> DPRNLPIRQQMEALIRRKQAEITQGLESIDTVKFHADTWTRGNDGGGGTSMVIQDGTTFEKGGVNVSVVYGQLSPAAVSAMKADHKNLRLPEDPKTGLPVTDGVKFFACGLSMVIHPVNPHAPTTHLNYRYFETWNQDGTPQTWWFGGGADLTPSYLYEEDGQLFHQLHKDALDKHDTALYPRFKKWCDEYFYITHRKETRGIGGIFFDDYDERD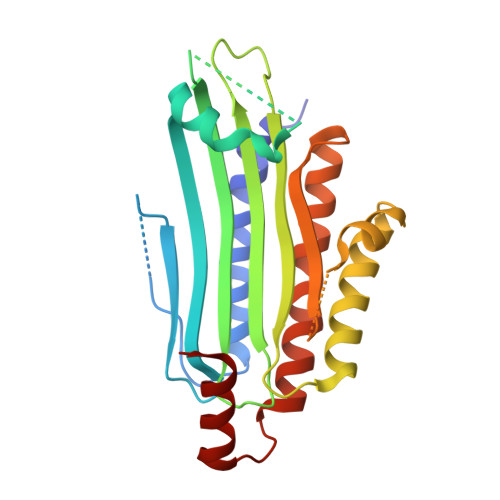PQEILKMVEDCFDAFLPSYLTIVKRRKDMPYTKEEQQWQAIRRGR> EPKFTKCRSPERETFSCHWTDEVHHGTKNLGPIQLFYTRRNTQEWTQEWKECPDYVSAGENSCYFNSSFTSIWIPYCIKLTSNGGTVDEKCFSVDEIVQPD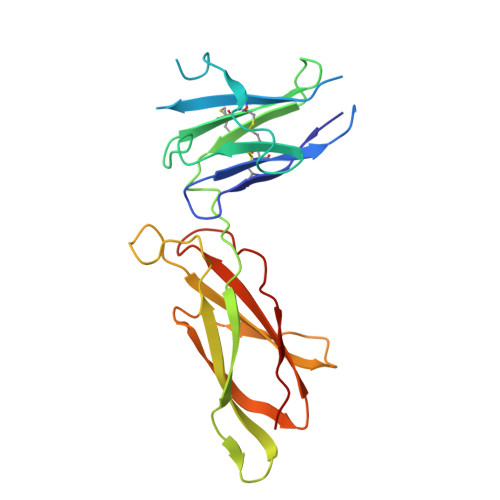PPIALNWTLLNVSLTGIHADIQVRWEAPRNADIQKGWMVLEYELQYKEVNETKWKMMDPILTTSVPVYSLKVDKEYEVRVRSKQRNSGNYGEFSEVLYVTLPQM> MATCAAVSLATAVFQVAAKYVNKARDAVASALPSPSNIDGVQQDWRQQVKELKKHTRVLGFVLPLAKAFAAESLTSVYARTFERAAFGFAKMYLFCLFMRVL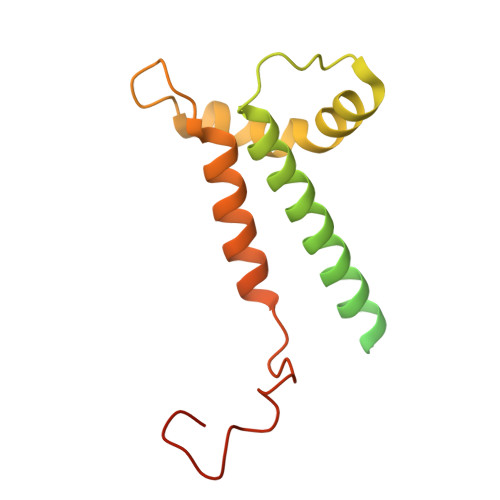LSWFPSIDWNSQPWAFLRLITEPYLQIYRGILPPLFGQLDFTPLFGFLILQDVVELMSPVYTLGHAKDTSMFWTTTDIMCYFDGH>CSLSPNLNIPEANYSIDNKLGALSWEKETNSSITKNWWKDFDDENLNKVVDLALKNNNDLKLAFIHMEQAAAQLGIDFSSLLPKFDGSASGSRAKTAINAPSNRTGEVSYGNDFKMGLNLSYEIDLWGKYRDTYRASKSGFKASEYDYEAARLSVISNTVQTYFNLVNAYENENALKEAYESAKEIYRINDEKFQVGAVGEYELAQARANLESMALQYNEAKLNKENYLKALKILTSNDLNDILYKNQSYQVFNLKEFDIPTGISSTILLQRPDIGSSLEKLTQQNYLVGVARTAFLPSLSL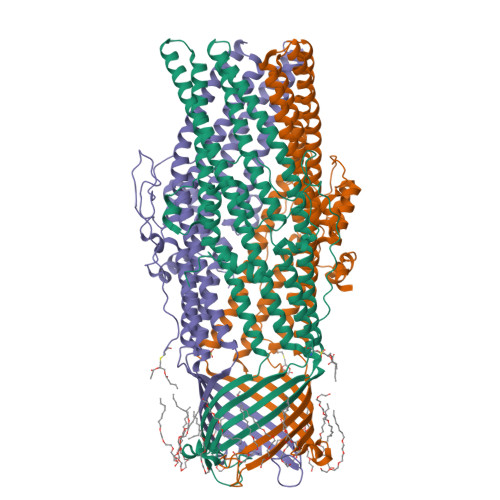TGLLGFESGDLDTLVKGGSKTWNIGGNFTLPIFHWGEIYQNVNLAKLNKDEAFVNYQNTLITAFGEIRYALVARKTIRLQYDNAQASEQSYKRIYEIAKERYDIGEMSLQDYLEARQNWLNAAVAFNNIKYSYANSIVDVIKAFGGGFEQSEDTSKNIKEESKNLDMSFREHHHHHH[3x]> MSQYSIQQSLGNASGVAVSPINADATLSTGVALNSSLWAGIGVFARGKPFTVLAVTESNYEDVLGEPLKPSSGSQFEPIRHVYEAIQQTSGYVVRAVPDDAKFPIIMFDESGEPAYSALPYGSEIELDSGEAFAIYVDDGDPCISPTRELTIETATADSAGNERFLLKLTQTTSLGVVTTLETHTVSLAEEAKDDMGRLCYLPTALEARSKYLRAVVNEELISTAKVTNKKSLAFTGGTNGDQSKISTAAYLRAVKVLNNAPYMYTAVLGLGCYDNAAITALGKICADRLIDGFFDVKPTLTYAEALPAVEDT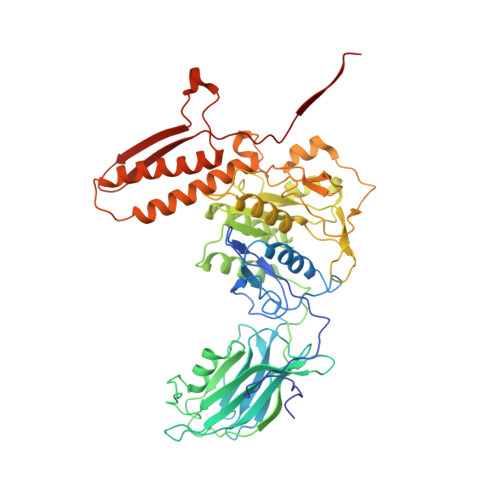GLLGTDYVSCSVYHYPFSCKDKWTQSRVVFGLSGVAYAAKARGVKKNSDVGGWHYSPAGEERAVIARASIQPLYPEDTPDEEAMVKGRLNKVSVGTSGQMIIDDALTCCTQDNYLHFQHVPSLMNAISRFFVQLARQMKHSPDGITAAGLTKGMTKLLDRFVASGALVAPRDPDADGTEPYVLKVTQAEFDKWEVVWACCPTGVARRIQGVPLLIK>MQDEQKRKEIVAEYFRKVNEGDVDAIVEMFTENATIEDPVGKDVREGRAAQREYFNSNVTAEVTIEPGHLSAGQDGKSVAVALAAEMTNILDPNRTRVKINAVDVFTLTPEGKIDSMRV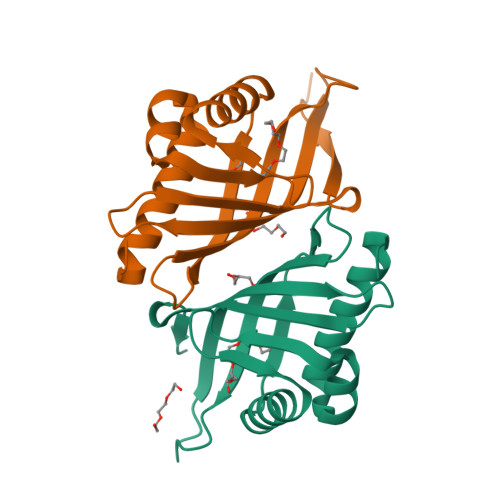FWGMTDIGVWNSSSVDKLAAALEHHHHHH[2x]> MAHHHHHHMGKNVVVLGTQWGDEGKGKIVDLLTQDAQVVVRYQGGHNAGHTLKINGVKTVLRLIPSGMLRPNVTCYIANGVVLSPQALLSEIKELEGNGINVRERLRISLACPLILPYHIALDKARETHMGKSAIGTTGRGIGPAYEDKVARRALRVGDLFHRDRFANKLTELLDYHNFVLTQYFKQPAVDLESLLGESLQWAEELRPMVCDVSACLHEHRKQGENILFEGAQGVYLDIDHGTYPYVTSSNTCVGSVINGAGFGPRYIDYVLGITKAYTTRVGGGPFPTELLDDVGKRIAERGQEFGAVTGRPRRCGWFDAVLLKRSIELNSISGLCVTKLDVLDGLEVLRIAVAYKDRDGNILSRPPLAADDFNDLLPVYEELPGWQESTADVTVMSDL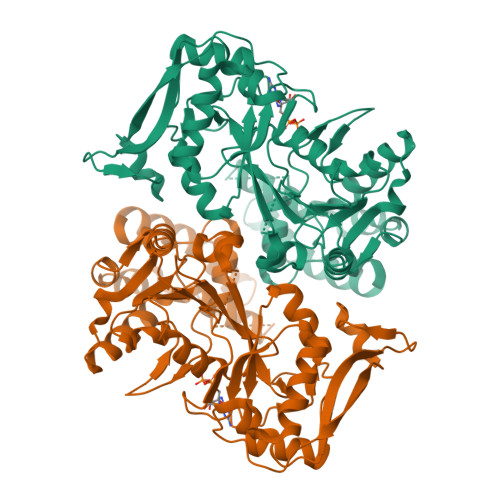PANARAYLKRIEEILGIPIDMLSTGPERDSTITLRGPFL> AEAGITGTWYNQLGSTFIVTAGADGALTGTYESAVGNAESRYVLTGRYDSAPATDGSGTALGWTVAWKNNYRNAHSATTWSGQYVGGAEARINTQWLLTSGTT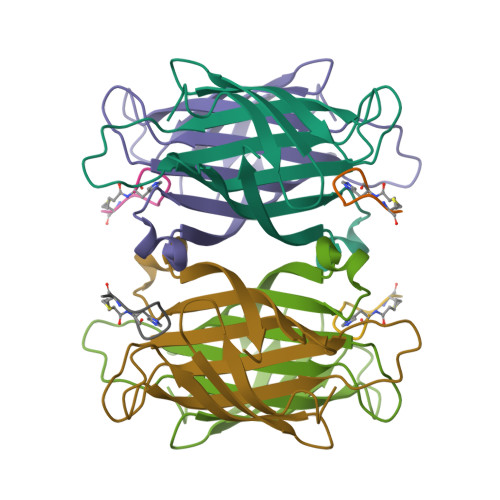EANAWKSTLVGHDTFTKVKP;> HPQGPPCKX> MAEPVSPLKHFVLAKKAITAIFDQLLEFVTEGSHFVEATYKNPELDRIATEDDLVEMQGYKDKLSIIGEVL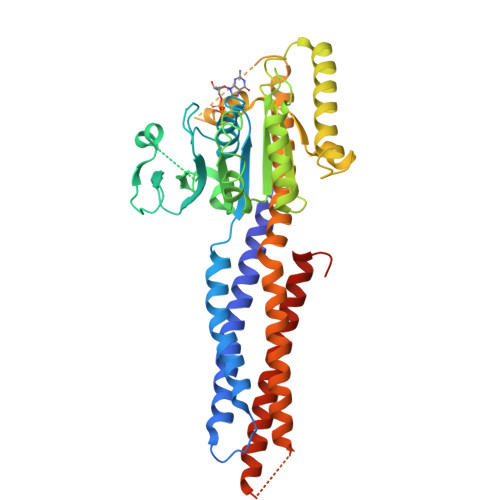SRRHMKVAFFGRTSSGKSSVINAMLWDKVLPSGIGHITNCFLSVEGTDGDKAYLMTEGSDEKKSVKTVNQLAHALHMDKDLKAGCLVRVFWPKAKCALLRDDLVLVDSPGTDVTTELDSWIDKFCLDADVFVLVANSESTLMNTEKHFFHKVNERLSKPNIFILNNRWDASASEPEYMEDVRRQHMERCLHFLVEELKVVNALEAQNRIFFVSAKEVLSARKQKAQGMPESGVALAEGFHARLQEFQNFEQIFEECISQSAVKTKFEQHTIRAKQILATVKNIMDSVNLAAEDGSGSGSGGSEIARLPKEIDQLEKIQNNSKLLRNKAVQLENELENFTKQFLPSSNEES>MHHHHHHHHDYKDDDDKLVPRGSEFMSDRPTARRWGKCGPLCTRENIMVAFKGVWTQAFWKAVTAEFLAMLIFVLLSLGSTINWGGTEKPLPVDMVLISLCFGLSIATMVQCFGHISGGHINPAVTVAMVCTRKISIAKSVFYIAAQCLGAIIGAGILYLVTPPSVVGGLGVTMVHGNLTAGHGLLVELIITFQLVFT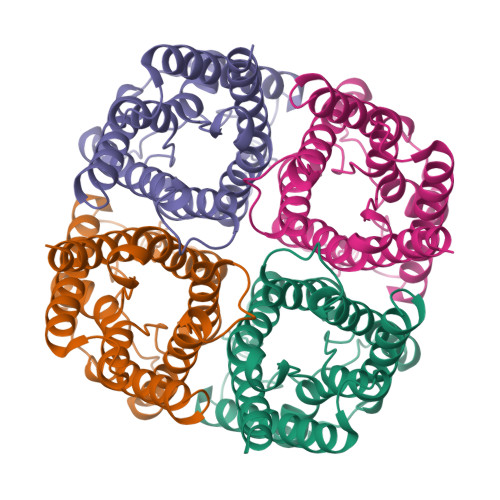IFASCDSKRTDVTGSIALAIGFSVAIGHLFAINYTGASMNPARSFGPAVIMGNWENHWIYWVGPIIGAVLAGGLYEYVFCPDVEFKRRFKEAFSKAAQQTKGSYMEVEDNRSQVETDDLILKPGVVHVIDVDRGEEKKGKDQSGEVLSSV[4x]> GPLGSMENSCNFNNSIKNVIVFYINEKALIEEKKMLSCYENKLLNLIKEDCENIMLKYKPNLSYICSLLKVDDTSEENIKHIKDQIIESLENDNRPSVKLAIISLISMIVEMNGYKGKNIPMSFLIEDIALKISENSEDLINF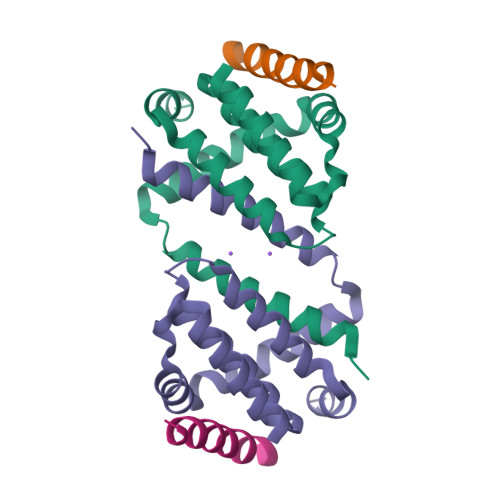INIKNKQKS;> DMRPEIWIAQELRRIGDEFNAYYARR Here, we conduct a comprehensive functional analysis of the Antibiotic_NAT family of aminoglycoside acetyltransferases. AG resistance is primarily conferred by three classes of aminoglycoside-modifying enzymes (AMEs): phosphotransferases (APHs), nucleotidylyltransferases (ANTs), and acetyltransferases (AACs). AMEs permanently alter the AG substrate, preventing them from binding to their target, the A-site of the 16S rRNA in the bacterial ribosome. The fold typical of the Antibiotic_NAT family is evident in all structures, composed of 13 α-helices and 8 β-strands, and determined structures superpose with pairwise RMSD’s 0.8–1.0 Å between 197 to 266 matching Cα atoms.

Notably, the meta-AAC0038 enzyme was also active against apramycin which inspired our structural analysis of this activity. Using the catalytically inactive His168Ala mutant of this enzyme, we were able to determine the crystal structures of ternary meta-AAC0038H168A•apramycin•CoA and the binary meta-AAC0038H168A•acetyl-CoA complexes. In line with the previously discussed Antibiotic_NAT enzyme structures, meta-AAC0038 accommodated the substrates in the negatively charged cleft formed by the minor subdomain, with the 3-N group of apramycin located within 2.6 Å of the sulfhydryl group of CoA. Notably, the I and III rings of apramycin were positioned out from the active site cleft and did not form interactions with the enzyme except for hydrogen bonds with the Asp94 and Asp162 sidechains. The ability to retain this AG molecule in the active site via very few contacts could explain the activity of meta-AAC0038 on this substrate resulting in the low-level resistance to apramycin which was not detected for the other representatives of Group 3 Antibiotic_NAT enzymes. According to our meta-AAC0038-apramycin complex structure, the binding of apramycin to this enzyme differed from its interactions to AAC(3)-IVa. The meta-AAC0038 and AAC(3)-IIIb structures superimpose with RMSD 0.54 Å across 219 Cα atoms, share all the minor subdomain structural elements, and show complete conservation of AG binding residues. However, the position corresponding to Glu223 in AAC(3)-IIIb is occupied by Asp213 in meta-AAC0038. Glu223 is positioned at the ring I binding site of apramycin, which may impact the ability of AAC(3)-IIIb to accommodate this AG as a substrate.

>VSSRVSTRSSLAEDLRAIGLADGDAVLVHAALRKVGKIVGGPDDILDAMRDVIGPAGTVLGYADWQLEDEIRDDPAMREHIPAFDPLRSRSIRDNGFWPELIRTTPGALRSASPGASMAAIGGEAEWFTADHALDYGYGPRSPLGKLVEAKGKVLMLGAPLDTMTLLAHAEHLADFPNKRILRYEAPILVDGEKVWRWFEEFDTSDPPDGLADDYFAGIVEEFLATGRGKRGKIGEASSVLVPADEIVAFAVDWLERWGRTAR[2x]>MGSDKIHHHHHHMIEYRIEEAVAKYREFYEFKPVRESAGIEDVKSAIEHTNLKPFATPDDIKKLCLEARENRFHGVCVNPCYVKLAREELEGTDVKVVTVVGFPLGANETRTKAHEAIFAVESGADEIDMVINVGMLKAKEWEYVYEDIRSVVESVKGKVVKVIIETCYLDTEEKIAACVISKLAGAHFVKTSTGFGTGGATAEDVHLMKWIVGDEMGVKASGGIRT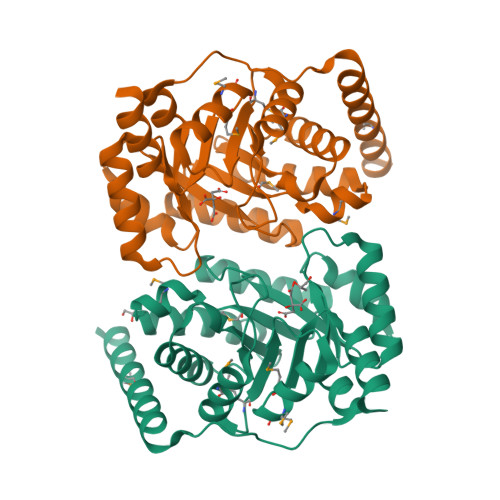FEDAVKMIMYGADRIGTSSGVKIVQGGEERYGG[2x]> MHHHHHHHAVRASEISRVYEAYPEKKATLYFLVLGFLALIVGSLFGPFQALNYGNVDAYPLLKRLLPFVQSYYQGLTLHGVLNAIVFTQLFAQAIMVYLPARELNMRPNMGLMWLSWWMAFIGLVVFALPLLANEATVLYTFYPPLKGHWAFYLGASVFVLSTWVSIYIVLDLWRRWKAANPGKVTPLVTYMAVVFWLMWFLASLGLVLEAVLFLLPWSFGLVEGVDPLVARTLFWWTGHPITYFWLLPAYAIIYTILPKQAGGKLVSDPMARLAFLLFLLLSTPVGFHHQFADPGIDPTWKMIHSVLTLFVAVPSLMTAFTVAASLEFAGRLRGGRGLFGWIRALPWDNPAFVAPVLGLLGFIPGGAGGIVNASFTLDYVVHNTAWVPGHFHLQVASLVTLTAMGSLYWLLPNLTGKPISDAQRRLGLAVV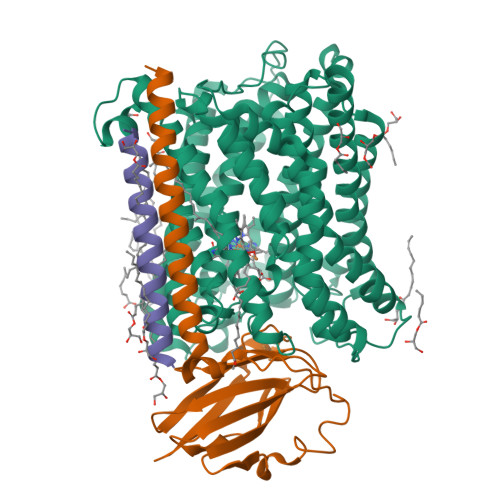WLWFLGMMIMAVGLHWAGLLNVPRRAYIAQVPDAYPHAAVPMVFNVLAGIVLLVALLLFIYGLFSVLLSRERKPELAEAPLPFAEVISGPEDRRLVLAMDRIGFWFAVAAILVVLAYGPTLVQLFGHLNPVPGWRLW;> MVDEHKAHKAILAYEKGWLAFSLAMLFVFIALIAYTLATHTAGVIPAGKLERVDPTTVRQEGPWADPAQAVVQTGPNQYTVYVLAFAFGYQPNPIEVPQGAEIVFKITSPDVIHGFHVEGTNINVEVLPGEVSTVRYTFKRPGEYRIICNQYCGLGHQNMFGTIVVKE;> MEEKPKGALAVILVLTLTILVFWLGVYAVFFARG>[2x]MTAAPAALHDRALHLLQTIWGYPAFRGVQGEIVQQVAEGGNALVLMPTGGGKSLCYQLPSLLRPGTGIVVSPLIALMKDQVDTLRQNGVRAAFLNSTLLPHEAREVEDALLRGDLDLLYVAPERLLMPRTLDLLERAPVALFAIDEAHCVSQWGHDFRPEYQQLSVLAERFPELPRVALTATADERTRADIKSVLRLEDAPQFVSSFDRPNIQYRVGLKDSPKTQLLHFIREEHPGDAGIVYCLSRKSVEETAKWLQAQGIDALAYHAGLSSTERNNVQERFLNEEGVIVCATVAFGMGIDKPNVRFVAHLDLPKSMEGYYQETGRAGRDGLPSTAWMVYGLSDVVNVRRMLAQSDAPEEVKRVEASKLDALLTYCEAATCRRQVLLHYFGEELSEPCGNCDVCLNPPRVRDLTREAQMALSATIRTGNRFGAAHLTDVLLGRETDKVLAQGHHQLPTFGVGKEHDEKLWRSVLRQLVSLGYLSADDHFGLRATGKSRGILKEGQKLLLREDTLLPGLEHHHHHH

RecQ helicases are a family of DNA strand-separating enzymes conserved from bacteria to humans that play a crucial role in the maintenance of genome stability. The helicase catalytic core is crucial for the ATPase and DNA-unwinding activities of these RecQ proteins. To better understand the structural and functional relationships of DrRecQ, we present crystal structures of the minimal helicase catalytic core from DrRecQ and its binary complex with ADP. The helicase catalytic core of DrRecQ contains four domains assembled in a trilobed or Y-shaped manner, with major clefts on its surface.

The apoenzyme structure was subsequently used to solve the binary complex structure with ADP at resolution of 2.90 Å. The nucleotide-binding pocket surrounded by conserved motifs is located at the D1 domain. Although we initially tried to model ATP into the experiment map, the γ-phosphate cannot fit well, suggesting that the ATP has been hydrolyzed to ADP during crystallization despite not adding a magnesium ion. ADP is bound with extensive interactions with the protein. The adenine moiety is sandwiched between Arg26 and Tyr22. The N6 and N7 atoms of the adenine ring are hydrogen-bonded to the side chain of Gln29, and the N6 atom is also situated within hydrogen-bonding distance of the main chain carbonyl oxygen atoms of Ala24. The ribosyl moiety is anchored via hydrogen bonds with the C-2 hydroxyl group of the side chain of Tyr22. The diphosphate is bound by backbone amides of motif I. ADP binding to the D1 domain causes slight alterations in motif I. The sequence alignment shows that motifs 0 (amino acids 16–29) and I (amino acids 45–53) are highly conserved in three RecQ proteins. Surprisingly, superposition of the apoenzyme against the binary complex reveals that the WH domain is positioned at a different orientation in these two structures, indicating the flexibility of the WH domain interdomain. The distinct domain orientation also indicates the interdomain flexibility of the WH domain. This motion generates a closed conformation in the binary complex structure and slightly enlarges the cleft between Zn-binding and WH domains in the apoform structure.>MAIPEEFDILVLGGGSSGSCIAGRLANLDHSLKVGLIEAGENNLNNPWVYLPGIYPRNMKLDSKTASFYTSNPSPHLNGRRAIVPCANVLGGGSSINFMMYTRGSASDYDDFQAEGWKTKDLLPLMKKTETYQRACNNPDIHGFEGPIKVSFGNYTYPVCQDFLRASESQGIPYVDDLEDLVTAHGAEHWLKWINRDTGRRSDSAHAFVHSTMRNHDNLYLICNTKVDKIIVEDGRAAAVRTVPSKPLNPKKPSHKIYRARKQIVLSCGTISSPLVLQRSGFGDPIKLRAAGVKPLVNLPGVGRNFQDHYCFFSPYRIKPQYESFDDFVRGDAEIQKRVFDQWYANGTGPLATNGIEAGVKIRPTPEELSQMDESFQEGYREYFEDKPDKPVMHYSIIAGFFGDHTKIPPGKYMTMFHFLEYPFSRGSIHITSPDPYAAPDFDPGFMNDERDMAPMVWAYKKSRETARRMDHFAGEVTSHHPLFPYSSEARALEMDLETSNAYGGPLNLSAGLAHGSW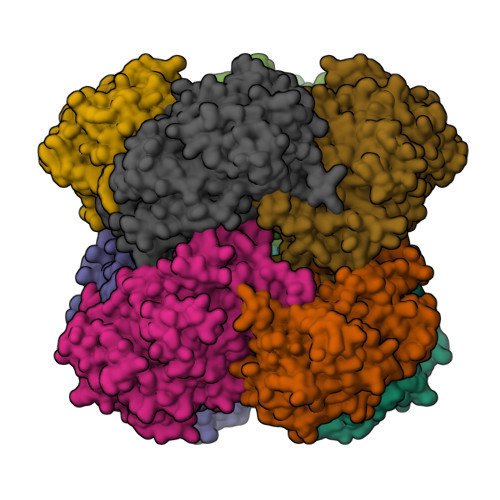TQPLKKPTAKNEGHVTSNQVELHPDIEYDEEDDKAIENYIREHTETTWHCLGTCSIGPREGSKIVKWGGVLDHRSNVYGVKGLKVGDLSVCPDNVGCNTYTTALLIGEKTATLVGEDLGYSGEALDMTVPQFKLGTYEKTGLARF[8x]>PVVIKTEGPAWTPLEPKLITRLADTVRTKGLRSPITMAEVEALMSSPLLPHDVTNLMRVILGPAPYALWMDAWGVQLQTVIAAATRDPRHPANGQGRGERTNLNRLKGLADGMVGNPQGQAALLRPGELVAITASALQAFREVARLAEPAGPWADIMQGPSESFVDFANRLIKAVEGSDLPPSARAPVIIDCFRQKSQPDIQQLIRT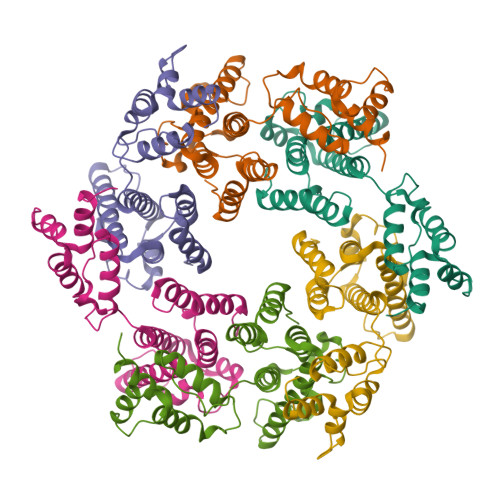APSTLTTPGEIIKYVLDRQKTA[3x]> YMIQEEEWDRDLLLDPAWEKQQRKTFTAWCNSHLRKAGTQIENIEEDFRNGLKLMLLLEVISGERLPKPDRGKMRFHKIANVNKALDYIASKGVKLVSIGAEEIVDGNVKMTLGMIWTIILRFAIQDISVEETSAKEGLLLWCQRKTAPYRNVNIQNFHTSWKDGLGLCALIHRHRPDLIDYSKLNKDDPIGNINLAMEIAEKHLDIPKMLDAEDIVNTPKPDERAIMTYVSCFYHAFAGAEQAETAANRICKVLAVNQENERLMEEYERLASELLEWIRRTIPWLENRTPAATMQAMQKKLEDFRDYRRKHKPPKVQEKCQLEINFNTLQTKLRISNRPAFMPSEGKMVSDIAGAWQRLEQAEKGYEEWLLNEIRRLERLEHLAEKFRQKASTHETWAYGKEQILLQKDYESASLTEVRALLRKHEAFESDLAAHQDRVEQIAAIAQELNELDYHDAVNVNDRCQKICDQWDRLGTLTQKRREALERMEKLLETIDQLHLEFAKRAAPFNNWMEGAMEDLQDMFIVHSIEEIQSLITAHEQFKATLPEADGERQSIMAIQNEVEKVIQSYNIRISSSNPYSTVTMDELRTKWDKVKQLVPIRDQSLQEELARQHANERLRRQFAAQANAIGPWIQNKMEEIARSSIQITGALEDQMNQLKQYEHNIINYKNNIDKLEGDHQLIQEALVFDNKHTNYTMEHIRVGWELLLTTIARTINEVETQILTRDAKGITQEQMNEFRASFNHFDRRKNGLMDHEDFRACLISMGYDLGEAEFARIMTLVDPNGQGTVTFQSFIDFMTRETADTDTAEQVIASFRILASDKPYILAEELRRELPPDQAQYCIKRMPAYSGPGSVPGALDYAAFSS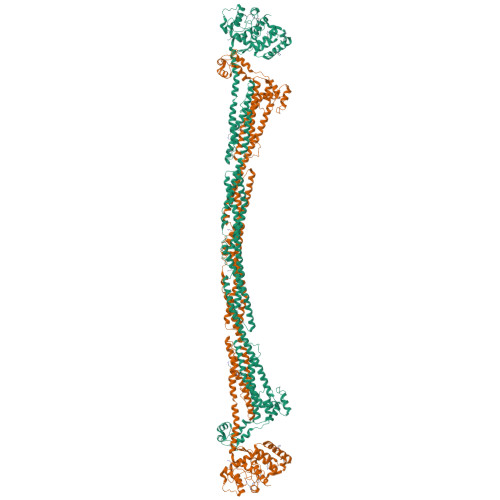ALYGESDL> MHHHHHHMPIIEQVRAREILDSRGNPTVEVEVALIDGTFARAAVPSGAATGEHEAVELRDGGDRYGGKGVQKAVQAVLDEIGPAVIGLNADDQ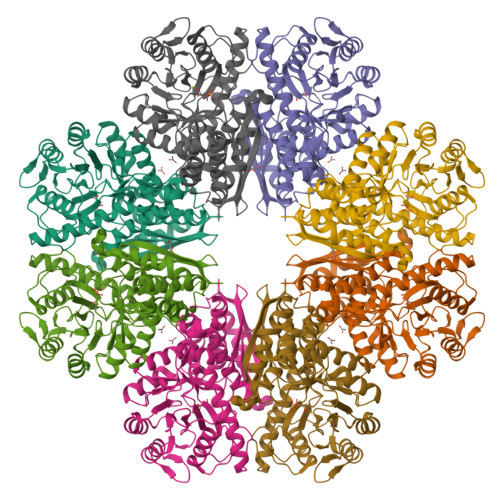RLVDQALVDLDGTPDKSRLGGNAILGVSLAVAKAAADSAELPLFRYVGGPNAHILPVPMMNILNGGAHADTAVDIQEFMVAPIGAPSFVEALRWGAEVYHALKSVLKKEGLSTGLGDEGGFAPDVAGTTAALDLISRAIESAGLRPGADVALALDAAATEFFTDGTGYVFEGTTRTADQMTEFYAGLLGAYPLVSIEDPLSEDDWDGWAALTASIGDRVQIVGDDIFVTNPERLEEGIERGVANALLVKVNQIGTLTETLDAVTLAHHGGYRTMISHRSGETEDTMIADLAVAIGSGQIKTGAPARSERVAKYNQLLRIEEALGDAARYAGDLAFPRFACETK> GPLGSEITSLDTENIDEILNNADVALVNFYADWCRFSQMLHPIFEEASDVIKEEFPNENQVVFAR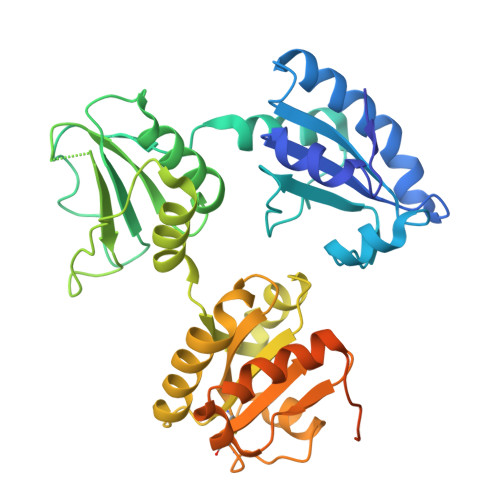VDCDQHSDIAQRYRISKYPTLKLFRNGMMMKREYRGQRSVKALADYIRQQKSDPIQEIRDLAEITTLDRSKRNIIGYFEQKDSDNYRVFERVANILHDDCAFLSAFGDVSKPERYSGDNIIYKPPGHSAPDMVYLGAMTNFDVTYNWIQDKCVPLVREITFENGEELTEEGLPFLILFHMKEDTESLEIFQNEVARQLISEKGTINFLHADCDKFRHPLLHIQKTPADCPVIAIDSFRHMYVFGDFKDVLIPGKLKQFVFDLHSGKLHREFHHGPDPTDTAPGEQAQDVASSPPESSFQKLAPSEYRYTLLRDRDEL>[2x]TGLRHRLDKVIDQLAIPALHTTVQYTGPLSVVDTVLANHAEAVLREAVSNAVRHANATSLAINVSVEDDVRVEVVDDGVGISGDITESGLRNLRQRADDAGGEFTVENMPTGGTL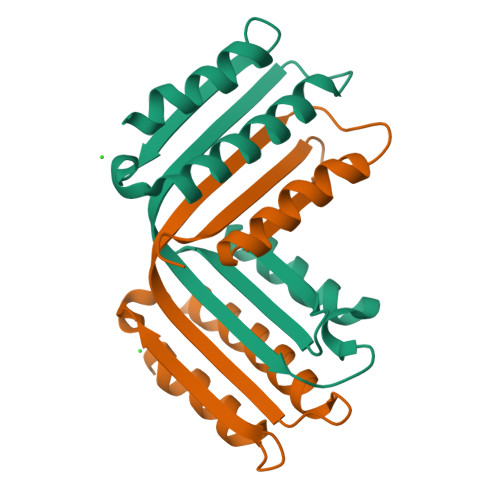LRWSAPLRL> MKAARLLFQSDRRTRHHMMIDGAINPREWFNWHPKEYQPWYFDRHKFIYEQGQYAAYNHLLCHQAYLKDIEHLTRYPEPRTFVIDCRMSPAKMHRWVPHSMWLPRDEVEYALQLTNDEFQEMYGFIKPAKDDDVILISHNGLASEQAGWEWRKQYYQHVYNYRGGTNELFGEDYQDFILKDRLDPWKGPYPQKS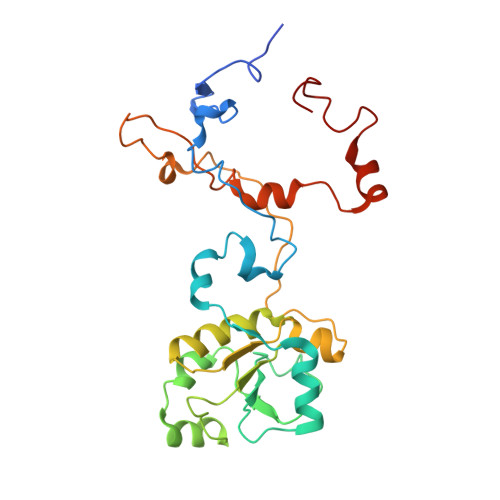IFVDKWSKRKVLTRTGPFDRQYEMQDFALPDLELERPRHSEDGPRQNMPYGLQ>RYILPSFIEHSSFGVKESNPYNKLFEERIIFLGVQVDDASANDIMAQLLVLESLDPDRDITMYINSPGGGFTSLMAIYDTMQYVRADIQTVCLGQAASAAAVLLAAGTPGKRMALPNARVLIHQPSLSGVIQGQFSDLEIQAAEIERMRTLMETTLARHTGKDAGVIRKDTDRDKILTAEEAKDYGIIDTVLEYRKLSAQTA[7x];>[7x]MRSNSQGLSLTDSVYERLLSERIIFLGSEVNDEIANRLCAQILLLAAEDASKDISLYINSPGGSISAGMAI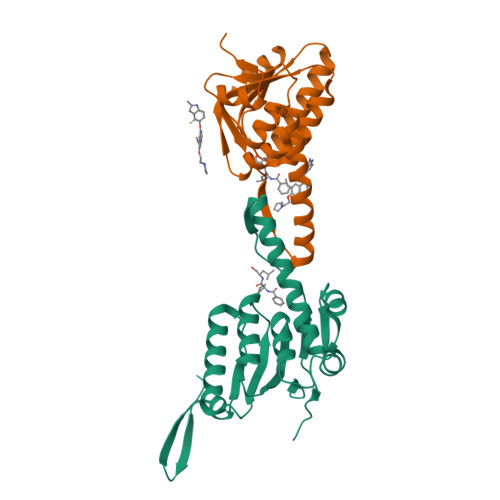YDTMVLAPCDIATYAMGMAASMGEFLLAAGTKGKRYALPHARILMHQPLGGVTGSAADIAIQAEQFAVIKKEMFRLNAEFTGQPIERIEADSDRDRWFTAAEALEYGFVDHIITRAHVNGEAQ> SGFVCNTCPEKWINFQRKCYYFGKGTKQWVHARYACDDMEGQLVSIHSPEEQDFLTKHASHTGSWIGLRDLDLEGEFIWVDGSHVDYSNWAPGEPNNGGQGEDCVMMRGSGRWNDAFCDRKLGAWVCDRLATCTPPASEGS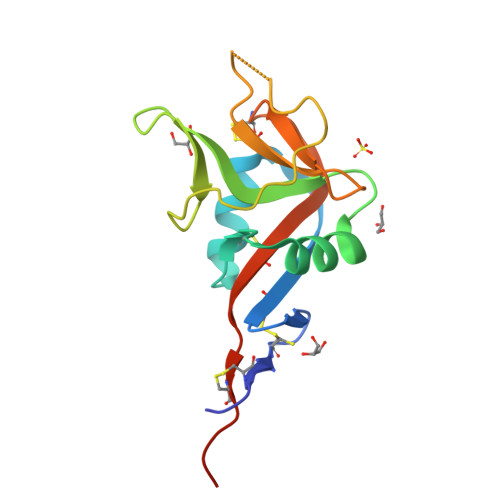AE>MANVNKVVRRRQVALLIALVLGIGAGGAGTWMVSEMNLKKAPPAK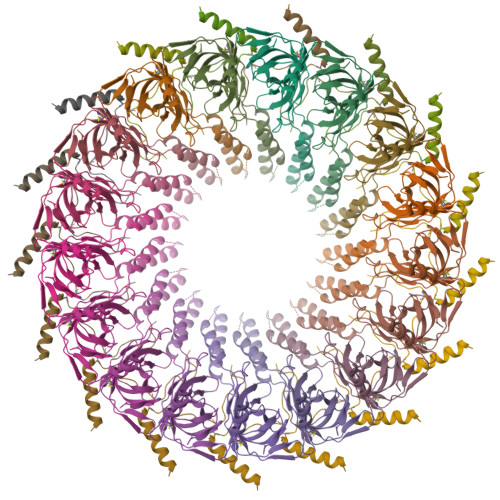APKGEPAPDMTGVVNQSFDNKVQRSAIAEAQRLNKETQTEIKKLRTEMGLVSRDLKGSQDRIRELEDQNQLLQTQLEAGKNFDSLSAEPLPGALASQGKPAPAGNVPPPTSFWPAGGGQAPAAPVMTPIQRPGMMDSQEFSLPDTGPKKPRFPWISSGSFVEAIVVEGADANASVTGDKNTAPMQLRLTGKVQMPNDEEFDLTGCFVTLEAWGDVSSERAIVRSRSISCKLGDDDIDQKIAGHVSFMGKNGIKGEVVMRNGQILLYAGGAGFLDGIGKGIEKASSTTVGVGATASMSAADIGQAGLGGGVSSAAKTLSDYYIKRAEQYHPVIPIGAGNEVTLVFQDGFQLETLEEARAKAAARKKQNQPSASSTPAAMPGNTPDMLKQLQDFRVGDTVDPATGQVVTQWSHPQFEK[17x];>[17x]MKKITLLLAGSALLLSGCAGVKSSFDCDATTSDTCMTMTKANQLARDKAAKQAGKPAAGGLPSLVNLPATSAVEVPSASRSAVTPPSGTRTVSTTPPVSAGTSAGVNTNTTTSTLTPRPVAGTPVTTTPSSVAYRPVVSVVTPTPSCQNVRCDNPGTVHPQRSRDQIATVWIAPWVDSDNAFHQPGRVSFVVSPADWVLPARVN>[9x]MKKIEAIIRPFKLDEVKIALVNAGIVGMTVSEVRGFGRQKGQTERY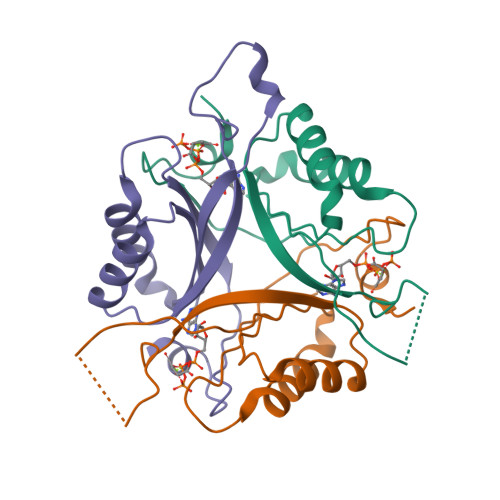RGSEYTVEFLQKLKLEIVVEDAQVDTVIDKIVAAARTGEIGDGKIFVSPVDQTIRIRTGEKNADAISAW> MSKKQKSKYIVIFGCGRLGSLIANLASSSGHSVVVVDKNEYAFHRLNSEFSGFTVVGDAAEFETLKECGMEKADMVFAFTNDDSTNFFISMNARYMFNVENVIA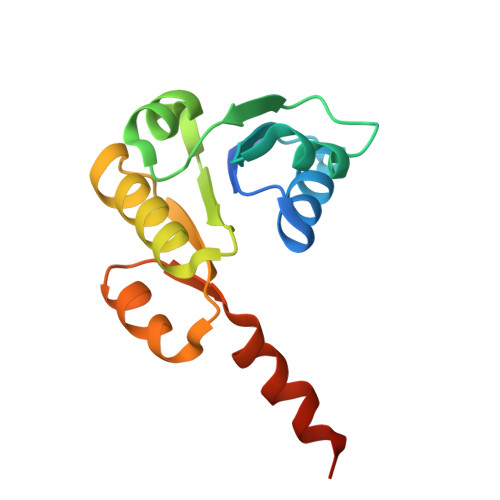RVYDPEKIKIFEENGIKTICPAVLMIEKVKEFIIGSEED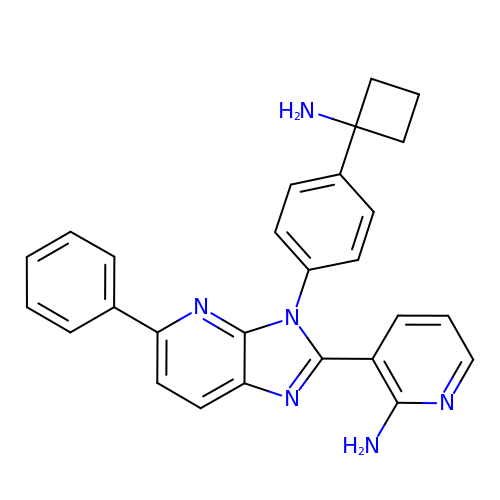3-[3-[4-(1-azanylcyclobutyl)phenyl]-5-phenyl-imidazo[4,5-b]pyridin-2-yl]pyridin-2-amine | C27 H24 N6 | HNFMVVHMKGFCMB-UHFFFAOYSA-N>[2x]GMTIKA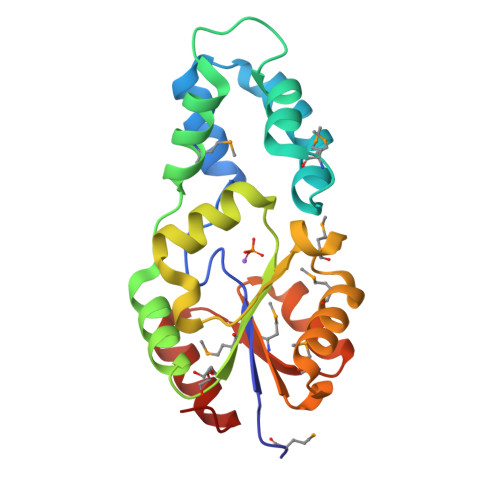LFWDIGGVLLTNGWDREQRADVAQRFGLDTDDFTERHRLAAPELELGRMTLAEYLEQVVFYQPRDFTPEDFRAVMEEQSQPRPEVLALARDLGQRYRMYSLNNEGRDLNEYRIRTFGLGEFLLAFFTSSALGVMKPNPAMYRLGLTLAQVRPEEAVMVDDRLQNVQAARAVGMHAVQCVDAAQLREELAALGVR>GMSGDSEVGTEAGLTLGGDGILRLTWPRGAAITAADAERAMLRVNQLCGDDRHPMLVDMATTADVSRGARAVFG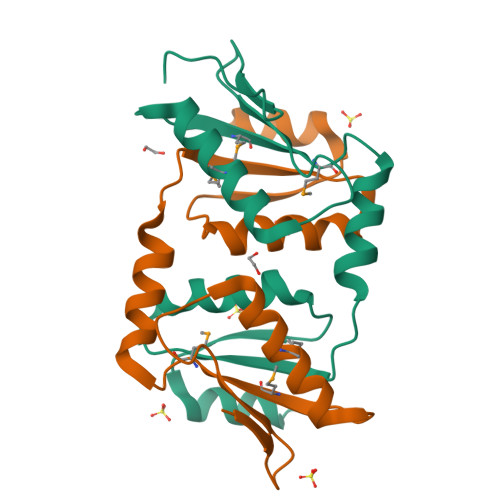RPCQASRIALLGSSPVDRVLANFFLGINAVPCPTKFFTSERDALTWLALT[2x]We describe here the high‐resolution crystal structures of GM from Clostridium cochlearium, reconstituted with AdoMeCbl and AdoEtCbl and the pseudo‐substrate (S,S)‐tartrate. As previously observed, GM forms a hetero‐tetramer consisting of two copies of the larger ϵ‐subunit (an (αβ)8 TIM‐barrel) and the smaller B12‐binding σ‐subunit, showing a typical Rossman fold. The ϵ‐subunit harbours the substrate‐binding site comprising three arginine residues (the “arginine claw”) that undergo strong polar binding interactions with the carboxylate groups of an (S,S)‐tartrate ion. The process catalysed by GM [12a] assigns the enzyme‐generated Ado‐radical the specific function of abstracting (in the direction from (S)‐glutamate to (2S,3S)‐3‐methylaspartate) the pro‐S H‐atom from the 4‐position of (S)‐glutamate, furnishing 5′‐deoxyadenosine and a 4‐glutamyl radical.

We have set out to test this AdoCbl‐activation hypothesis with two “stretched” AdoCbl‐homologues, designed and synthesised as potential structural mimics of “activated” AdoCbl, provisionally named “homocoenzyme B12” (AdoMeCbl) and “bis‐homocoenzyme B12” (AdoEtCbl). AdoMeCbl and AdoEtCbl are bound in a base‐off/His‐on form, with distances between cobalt and the coordinating histidine imidazole of 2.21 Å and 2.17 Å, respectively, similar to GM‐bound AdoCbl (2.22 Å) and free AdoMeCbl (2.19 Å). In both new structures, the electron density for the “stretched” AdoCbl‐homologues indicated an intact bond between the cobalt ion and the terminal carbons C6′ or C7′ of the 5′‐methyl‐ or 5′‐ethyl‐adenosyl ligands of AdoMeCbl and AdoEtCbl, respectively. The refined Co−C bond lengths at 2.07 Å or 1.98 Å for the bound AdoMeCbl and AdoEtCbl, respectively, were somewhat longer or slightly shorter than the 2.00 Å observed in the crystal structures of AdoCbl and AdoMeCbl, [25a] but in stark contrast to distances of >3.2 Å observed between cobalt and C5′ of the adenosyl ligand in GM reconstituted with AdoCbl. The distances from Co to C5′ of the Ado moieties of the bound AdoMeCbl and AdoEtCbl were 3.2 Å and 4.2 Å, strikingly comparable to the distances between the Co‐atom and C5′ in the two observed structures of “activated” AdoCbl in the crystal structure of GM reconstituted with AdoCbl. In GM‐AdoMeCbl, the cobalt‐bound AdoMe‐ligand fills the adenosine binding cavity with little strain, and its Co−C bond remains intact. However, in GM‐AdoMeCbl, the corresponding ribose unit of AdoMeCbl exhibits a 2T3 (2,3‐twist) conformation, similar to the particular 2E (C2′‐endo) ra‐conf in GM‐AdoCbl. Hence, AdoMeCbl is bound to GM with not only an intact Co−C bond but also exhibits the typical hallmarks of a rather unstrained ribose moiety. The experimental geometric parameters reflect only a minor “pull” in the case of AdoMeCbl and an opposite small “squeeze” in AdoEtCbl.

>[2x]MEKKTIVLGVIGSDCHAVGNKILDHAFTNAGFNVVNIGVLSPQENFIKAAIETKADAILVSSLYGQGEIDCKGLRQKCDEAGLEGILLYVGGNIVVGKQHWPDVEKRFKDMGYDRVYAPGTPPEVGIADLKKDLNIE;>[2x]MELKNKKWTDEEFHKQREEVLQQWPTGKEVDLQEAVDYLKKIPAEKNFAEKLVLAKKKGITMAQPRAGVALLDEHIELLRYLQDEGGADFLPSTIDAYTRQNRYDECENGIKESEKAGRSLLNGFPGVNHGVKGCRKVLEAVNLPLQARHGTPDSRLLAEIIHAGGWTSNEGGGISYNVPYAKNVTIEKSLLDWQYCDRLVGFYEEQGVHINREPFGPLTGTLVPPSMSNAVGITEALLAAEQGVKNITVGYGECGNMIQDIAALRCLEEQTNEYLKAYGYNDVFVTTVFHQWMGGFPQDESKAFGVIVTATTIAALAGATKVIVKTPHEAIGIPTKEANAAGIKATKMALNMLEGQRMPMSKELETEMAVIKAETKCILDKMFELGKGDLAIGTVKAFETGVMDIPFGPSKYNAGKMMPVRDNLGCVRYLEFGNVPFTEEIKNYNRERLQERAKFEGRDVSFQMVIDDIFAVGKGRLIGRPE> WVQPITAQKPSLTLWLDDKMFTGLINTGADVTII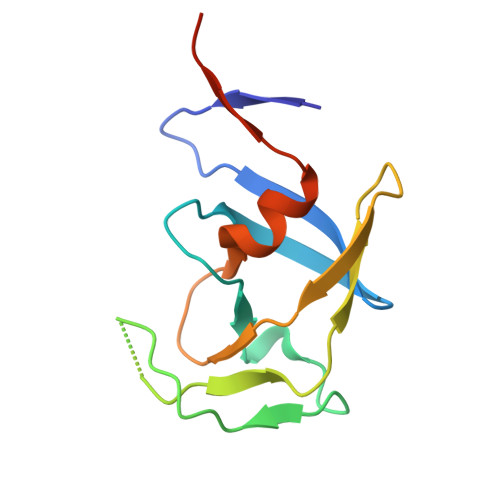KLEDWPPNWPITDTLTNLRGIGQSNNPKQSSKYLTWRDKENNSGLIKPFVIPNLPVNLWGRDLLSQMKIMMASPNDIVTA>NPPMFSQDVFSVTLREDVPPGFSVLQVTATDQDEGVNAEITYAFHNVDEQVERIFNLDKRTGEITTKDNLDFETAKSYTLNVEAKDPGDLASHCSIQVKILDENDCVPEVIVTSVFTPLPEDSPLGTVIALIKTRDRDSGENGDVYCHVLGNEGFVLKSSSKNYYKLVTDRTLDREAIPEYNVTIVAADRGKPPLSSNVIITLHISDVNDNAPVFHQASYLVHVAENNPPGTSIAQVSASDPDLGSNGLISYSIIASDLEPRALSSFVSVNQDSGVVFAQRAFDHEQLRSFQLTLQARDHGSPTLSANVSMRVLVGDRNDNAPRVLYPTLEPDGSALFDMVPRAAEPGYLVTKVVAVDADSGHNAWLSYHVLQASDPGLFSLGLRTGEVRTARALGDRDSARQRLLVAVRDGGQPPLSATATLHLIFADSLQEHHHHHHHH[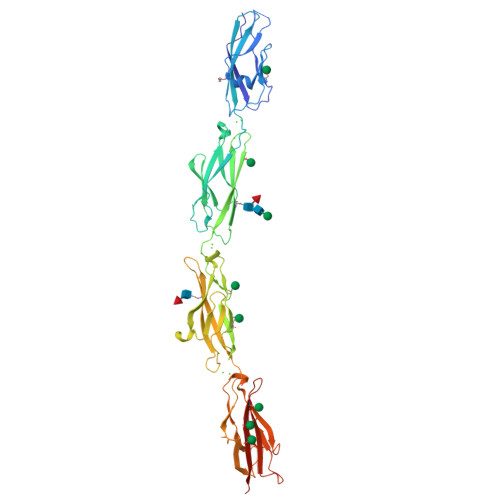3x]2-HYDROXYMETHYL-5-(6-METHYLSULFANYL-PURIN-9-YL)-TETRAHYDRO-FURAN-3,4-DIOL 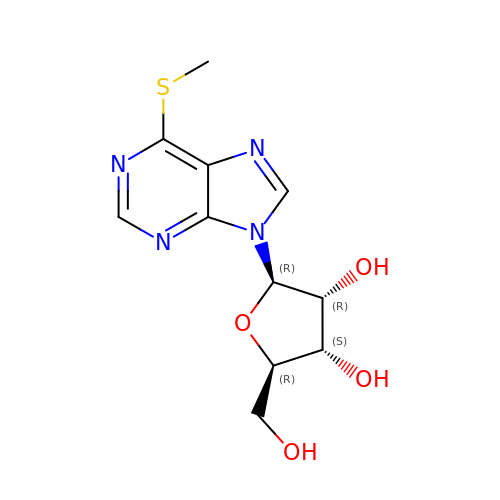| C11 H14 N4 O4 S | ZDRFDHHANOYUTE-IOSLPCCCSA-N>[2x]MAEIP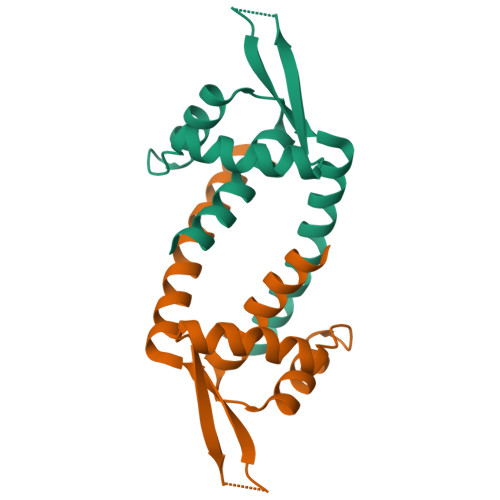KEMLRAQTNVILLNVLKQGDNYVYGIIKQVKEASNGEMELNEATLYTIFKRLEKDGIISSYWGDESQGGRRKYYRLTEIGHENMRLAFESWSRVDKIIENLEANKKSEAIK> MEKLGVEPEEEGGGDDDEEDAEAWAMELADVGAAASSQGVHDQVLPTPNASSRVIVHVDLDCFYAQVEMISNPELKDKPLGVQQKYLVVTCNYEAGKLGVKKLMNVRDAKEKCPQLVLVNGEDLTRYREMSYKVTELLEEFSPVVERLGFDENFVDLTEMVEKRLQQLQSDELSAVTVSGHVYNNQSINLLDVLHIRLLVGSQIAAEMREAMYNQLGLTGCAGVASNKLLAKLVSGVFKPNQQTVLLPESCQHLIHSLNHIKEIPGIGYKTAKCLEALGINSVRDLQTFSPKILEKELGISVAQRIQKLSFGEDNSPVILSGPPQSFSEEDSFKKCSSEVEAKNKIEELLASLLNRVCQDGRKPHTVRLIIRRYSSE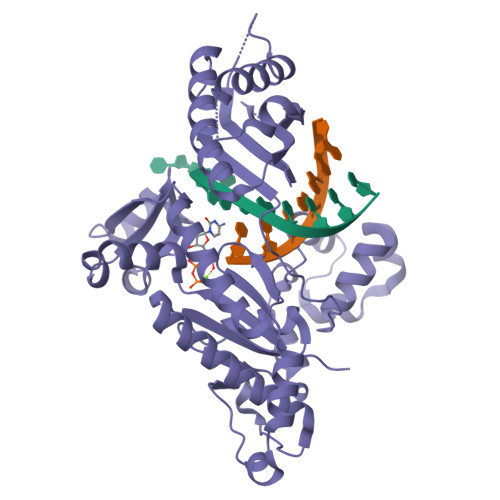KHYGRESRQCPIPSHVIQKLGTGNYDVMTPMVDILMKLFRNMVNVKMPFHLTLLSVCFCNLKALNTAK> APAILLVDDEPHSLAAMKLALEDDFDVLTAQGAEAAIAILEEEWVQVIICDQRMPGRTGVDFLTEVRE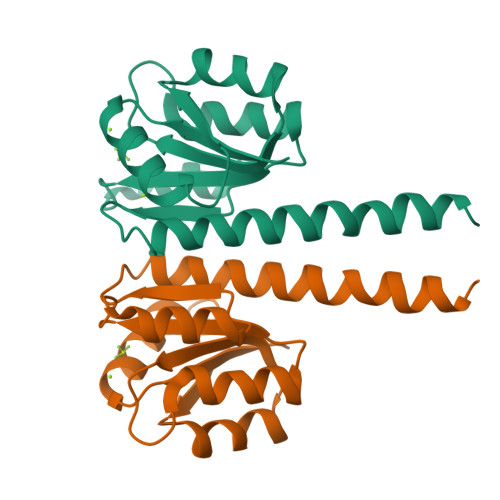RWPETVRIIITGYTDSASMMAAINDAGIHQFLTKPWHPEQLLSSARNAARMFTLARENERLSLEMRLLERP>MGAAILPDLGTEILIPVCAVIGIAFALFQWLLVSKVKLSAVRDASPNAAAKNGYNDYLIEEEEGINDHNVVVKCAEIQNAISEGATSFLFTEYKYVGIFMVAFAILIFLFLGSVEGFSTSPQACSYDKTKTCKPALATAIFSTVSFLLGGVTSLVSGFLGMKIATYANARTTLEARKGVGKAFITAFRSGAVMGFLLAANGLLVLYIAINLFKIYYGDDWGGLFEAITGYGLGGSSMALFGRVGGGIYTKAADVGADLVGKVERNIPEDDPRNPAVIADNVGDNVGDIAGMGSDLFGSYAESSCAALVVASISSFGLNHELTAMLYPLIVSSVGILVCLLTTLFATDFFEIKAVKEIEPALKKQLVISTVLMTIGVAVVSFVALPTSFTIFNFGVQKDVKSWQLFLCVAVGLWAGLIIGFVTEYYTSNAYSPVQDVADSCRTGAATNVIFGLALGYKSVIIPIFAIAISIFVSFTFAAMYGIAVAALGMLSTIATGLAIDAYGPISDNAGGIAEMAGMSHRIRERTDALDAAGNTTAAIGKGFAIGSAALVSLAMFGAFVSRASITTVDVLTPKVFIGLIVGAMLPYWFSAMTMKSVGSAALKMVEEVRRQFNTIPGLMEGTAKPDYATCVKISTDASIKEMIPPGALVMLTPLVVGILFGVETLSGVLAGSLVSGVQIAISASNTGGAWDNAKKYIEAGASEHARSLGPKGSDCHKAAVIGDTIGDPLKDTSGPSLNILIKL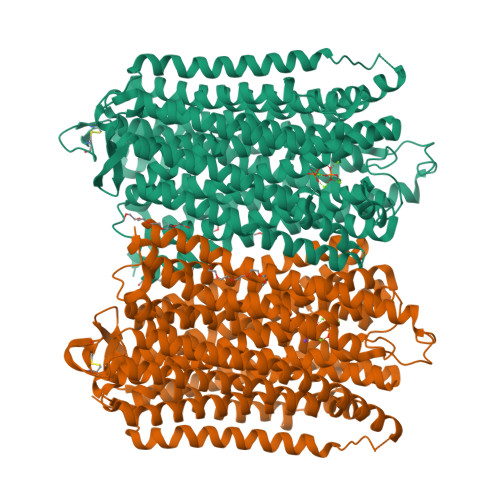MAVESLVFAPFFATHGGLLFKIF[2x]> GMSSKEEILSILEAFASTERMGSFFLDNATADFLFIRPSGN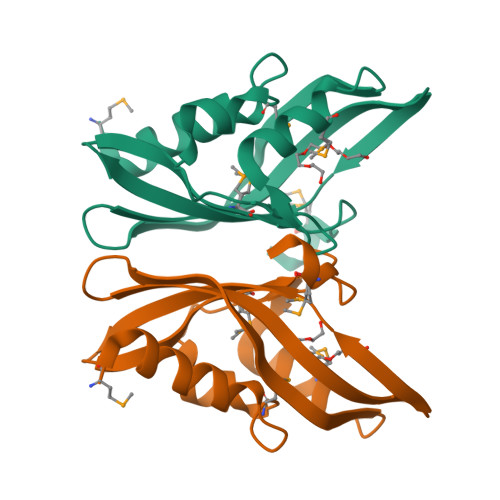PLDAKGFENMWSSGDLVLESAEITKVHKFELLGSNAAICVFTLGSKFTYKGTQNDDLPTVTSIFKKIDEKWKVAWMQRSSGQSDMTLWNE> GALERLPDGPRIHVPRKTALRPTVARQVFQPAFAPAVLSKFDPRTDADVDEVAFSKHTSNQETLPPVFRMVAREYANRVFALLGRDNGRLSVKQALDGLEGMDPMDKNTSPGLPYTTLGMRRTDVVDWETATLIPFAAERLEKMNNKDFSDIVYQTFLKDELRPIEKVQAAKTRIVDVPPFEHCILGRQLLGKFASKFQTQPGLELGSAIGCDPDVHWTAFGVAMQGFERVYDVDYSNFDSTHSVAMFRLLAEEFFSEENGFDPLVKDYLESLAISKHAYEEKRYLITGGLPSGCAATSVLNTIMNNIIIRAGLYLTYKNFEFDDVKVLSYGDDLLVATNYQLNFDRVRTSLAKTGYKITPANKTSTFPLESTLEDVVFLKRKFKKEGPLYRPVMNREALEAMLSYYRPGTLSEKLTSITMLAVHSGKQEYDRLFAPFREVGVIVPTFESVEYRWRSL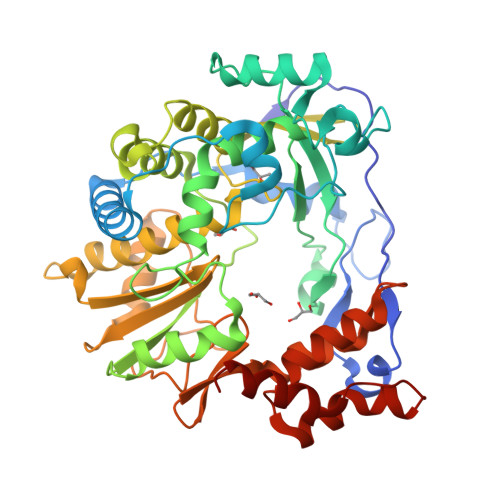FW> MAISIKTPEDIEKMRVAGRLAAEVLEMIEPYVKPGVSTGELDRICNDYIVNEQHAVSACLGYHGYPKSVCISINEVVCHGIPDDAKLLKDGDIVNIDVTVIKDGFHGDTSKMFIVGKPTIMGERLCRITQESLYLALRMVKPGINLREIGAAIQKFVEAEGFSVVREYCGHGIGQGFHEEPQVLHYDSRETNVV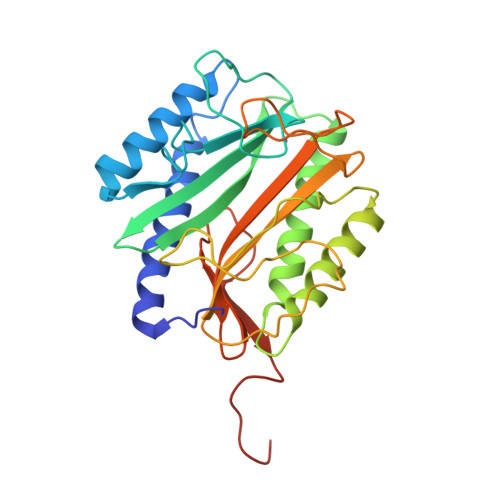LKPGMTFTIEPMVNAGKKEIRTMKDGWTVKTKDRSLSAQYEHTIVVTDNGCEILTLRKDDTIPAIISHDELVPRGSLEHHHHHH> MIRDIIRMGDKRLLRVAPQVTNLGSAELHALV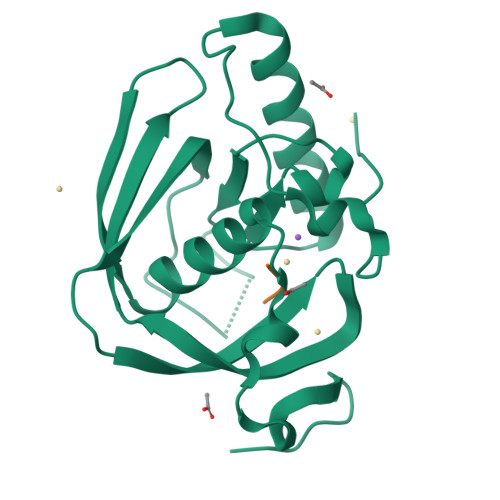SDMFETMGAAHGVGLAAPQIAVDLQLMVFGFEASERYPEAPAVPLTALANAQIEPLSDEMENGWEGCLSIPGLRAVIPRYRYIRYRGFAPDGSPIEREAEGFHARVVQHEYDHLVGRLYPSRIENFDTFGFDDVLSYDL;> MAS> GSSRAMGNEVAGVEDISVEITPSSKRNSDARRTSRNCSSNEERKRRKYFHMLYLVCLMVHGFIRNEWINSKRLSRKL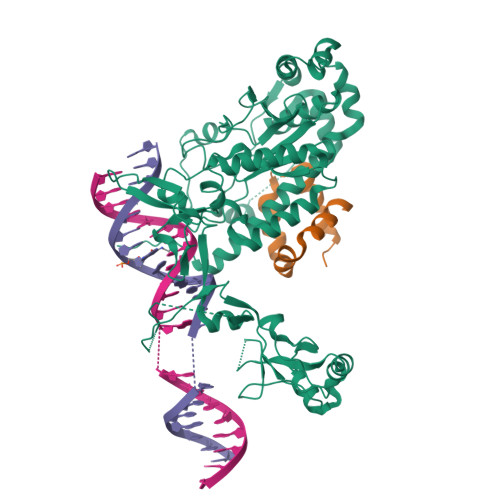SNLVPEKVFELLHPQKDEELPLRSTRKLLDGLKKCMELWQKHWKITKKYDNEGLYMRTWKEIEMSANNKRKFKTLKRSDFLRAVSKGHGDPDISVQGFVAMLRACNVNARLIMSCQPPDFTNMKIDTSLNGNNAYKDMVKYPIFWCEVWDKFSKKWITVDPVNLKTIEQVRLHSKLAPKGVACCERNMLRYVIAYDRKYGCRDVTRRYAQWMNSKVRKRRITKDDFGEKWFRKVITALHHRKRTKIDDYEDQYFFRRDESEGIPDSVQDLKNHPYYVLEQDIKQTQIVKPGCKECGYLKVHGKVGKVLKVYAKRDIADLKSARQWYMNGRILKTGSRCKKVIKRTVGRPKGEAEEEDERLYSFEDTELYIPPLASASGEITKNTFGNIEVFAPTMIPGNCCLVENPVAIKAARFLGVEFAPAVTSFKFPVLSGIVVAKWLREAIETAIDGIEFI;> GSGNASSGALGTTGGATDAAQGGPPGSIGLTVEDLLSLRQVVSGNPEALAPLLENISARYPQLREHIMANPEVFVSMLLEAVGDNMQDVMEGADDMVEGEDIEVTGEAAAAGLGQGEGEGSFQVDYTPEDDQAISRLCELGFERDLVIQVYFACDKNEEAAANILFSDHAD> MRCTRAIRQTARTGWLTWLAILAVTAPVTSPAWADDPPATVYKYDSRPPEDVFQNGFTAWGNNDNVLEHLTGRSCQVGSSNSAFVSTSSSRRYTEVYLEHRMQEAVEAERAGRGTGHFIGYIYEVRADNNFYGAA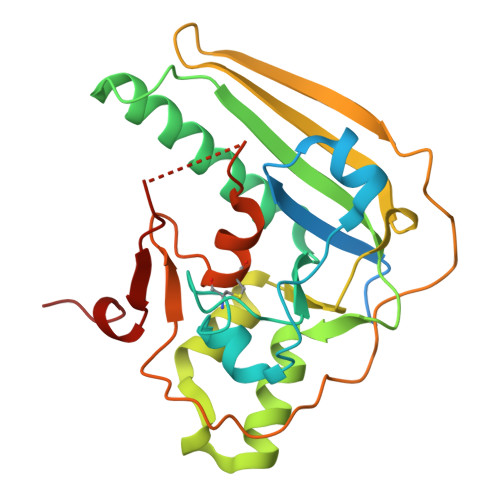SSYFEYVDTYGDNAGRILAGALATYQSGYLAHRRIPPENIRRVTRVYHNGITGETTTTEYSNARYVSQQTRANPNPYTSRRSVASIVGTLVRMAPVVGACMARQAESSEAMAAWSERAGEAMVLVYYESIAYSF>[2x]MDKTVTLATVGTTNPFSY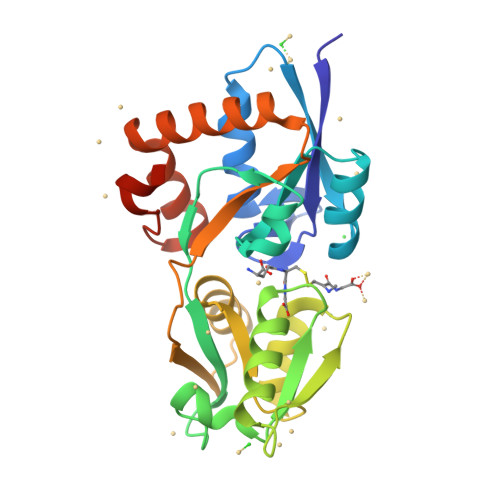EKKGKLTGYDIEVAKEVFKASDKYDVKYQKTEWTSIFSGLDSDKYQIGANNISYTKERANKYLYSNPTASNPLVLVVPKDSDIKSYNDIAGHSTQVVQGNTTVPMLQKFNKNHENNQVKLNFTSEDLAHQIRNVSDGKYDFKIFEKISAETIIKEQGLDNLKVIDLPSDQKPYVYFIFAQDQKDLQKFVNKRLKKLYENGTLEKLSKKYLGGSYLPDKKDMKLEHHHHHH>[2x]SNAQEEKLPKILIVEDDERLARLTQEYLIRNGLEVGVETDGNRAIRRIISEQPDLVVLDVMLPGADGLTVCREVRPHYHQPILMLTAR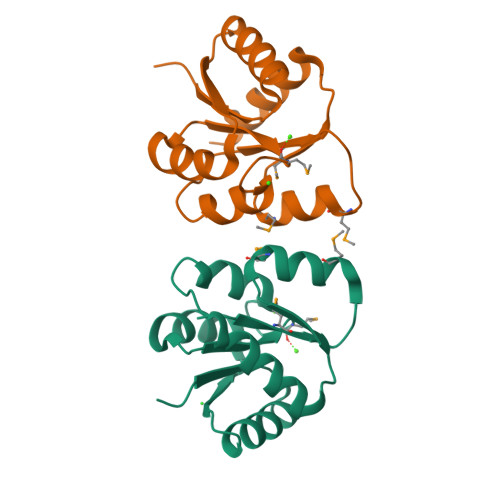TEDMDQVLGLEMGADDYVAKPVQPRVLLARIRALLRRT>[2x]EARPKIGLVLSGGAARGLAHIGVLKALDEQGIQIDAIAGTSMGAVVGGLYASGYTPAELERIALEMDWQQA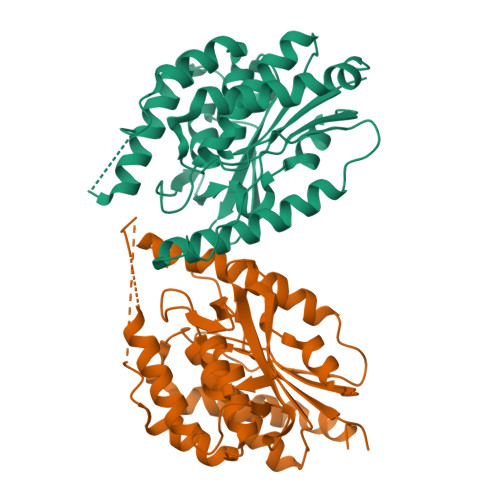LSDAPPRKDVPFRRKQDDRDFLVKQKISFRDDGTLGLPLGVIQGQNLAMVLESLLVHTSDNRDFDKLAIPFRAVSTDIATGEKVVFRKGHLPQAIRASMSIPAVFAPVEIDGRLLVDGGMVDNIPVDVARDMGVDVVIVVDIGNPLRDRKDLSTVLDVMNQSITLMTRKNSEAQLATLKPGDVLIQPPLSGYGTTDFGRVPQLIDAGYRATTVLAARLAELRKPKDLNSEALDVARTPNQRKP> SNLNPNAAEFVPGVKY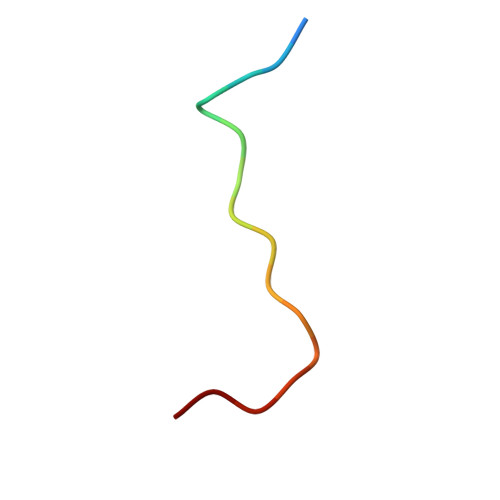G> PVLNLNDPQAVERYEEFMRQSPYGQVTQDLGWAKVMNNWEPVDVYLEDDQGAIIAAMSMLLGDTPTDKKFAYASKGPVMDVTDVDLLDRLVDEAVKALDGRAYVLRFDPEVAYSDEFNTTLQDHGYVTRNRNVADAGMHATIQPRLNMVLDLTKFPDAKTTLDLYPSKTKSKIKRPFRDGVEVHSGNSATELDEFFKTYTTMAERHGITHRPIEYFQRMQAAFDADTMRIFVAEREGKLLSTGIALKYGRKIWYMYAGS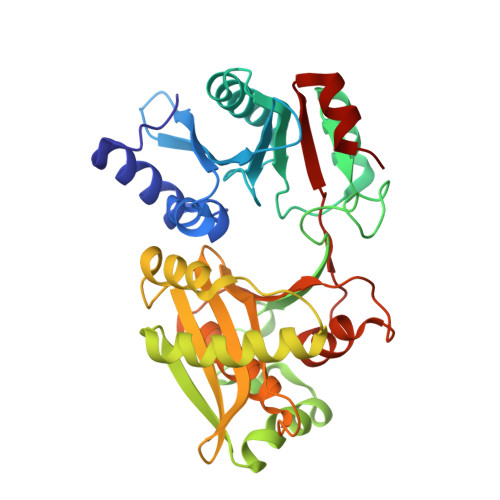MDGNTYYAPYAVQSEMIQWALDTNTDLYDLGGIESESTDDSLYVFKHVFVKDAPREYIGEIDKVLDPEVYAELVKD> QLDD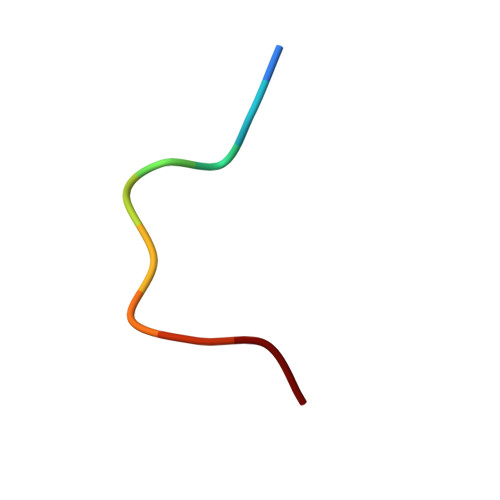FIDGIF> XQWVRE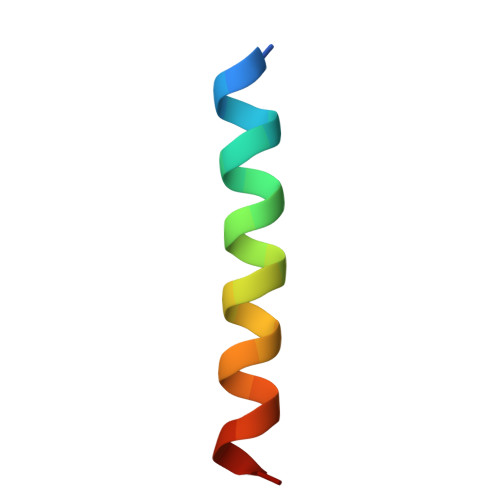IAAGLRRAADDVNAQVERX>[4x]AGITGTWYNQLGSTFIVTAGADGALTGTYESATSNEIKRYVLTGRY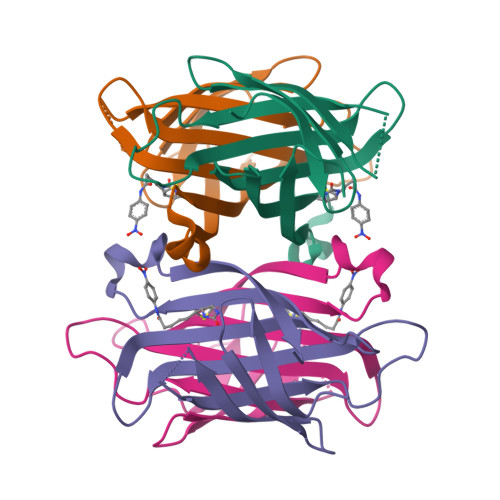DSAPATDGSGTALGWTVAWKNNYRNAHSATTWSGQYVGGAEARINTQWLLTSGTTEANAWKSTLVGHDTFTKVKP>[2x]MSNAALATAPHALELDVHPVAGRIGAEIRGVKLSPDLDAATVEAIQAALVRHKVIFFRGQTHLDDQSQEGFAK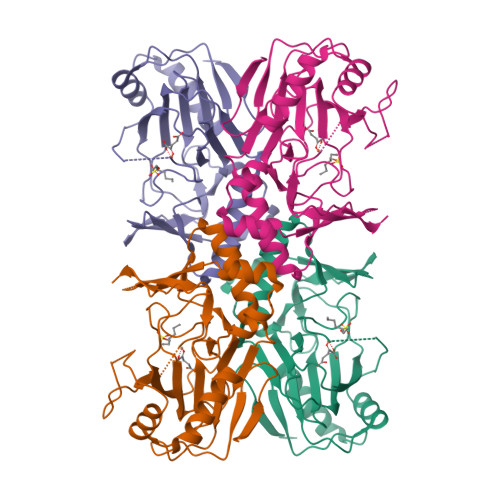LLGEPVAHPTVPVVDGTRYLLQLDGAQGQRANSWHTDVTFVEAYPKASILRSVVAPASGGDTVWANTAAAYQELPEPLRELADKLWAVHSNRYDYASLKPDIDPAKLERHRKVFTSTVYETEHPVVRVHPISGERALQLGHFVKRIKGYSLADSQHLFAVLQGHVTRLENTVRWRWEAGDVAIWDNRATQHYAVDDYGTQPRIVRRVTLAGEVPVGVDGQLSRTTRKG>MTDFDSLSGTSTTWVNELGSVMTIDVDRKGGVTGYYVNNAPGTGCRGLPYDLSGHAHGSTIAFSVVWSNGIADCRSATSWAGYARKTFGGGVQIVTQWSLAFV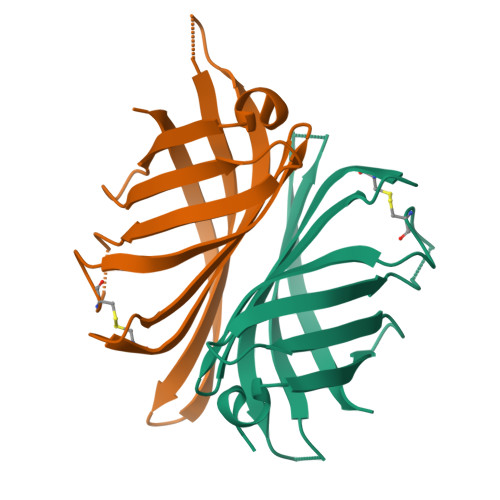GKAGGKIETGQNVFTYQAYDAQPSPADK[4x]>PSVYDAAAQLTADVKKDLRDSWKVIGSDKKGNG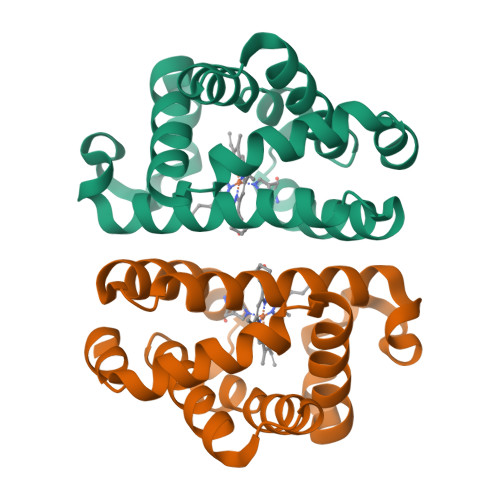VALVTTLFADNQETIGYFKRLGDVSQGMANDKLRGHSITLMYALQNFIDQLDNPDDLVCVVEKFAVNHITRKISAAEFGKINGPIKKVLASKNFGDKYANAWAKLVAVVQAAL[2x]> GAMGMNGIDDLLNINDRIKQVQNERNELASKLQNLKQSLASNDTGGGSGGGSDSSDLLQREAILANELNILDNLKTFLNLIKEVKTNLNILELENCYYSLQSLRKKMRNNAAYLKQSFNFQQSISTYVDTLHLELVSTLYKILTNGFWKITENSIQFTPTVEWGKDKVHIEYDTFMDFVAQQYFPKGSLDNQAWFILDMTSADSQEQVRAKLNTIMKEYMNLSRIVSMIKNSIFISGKEISYENEKNILVFSKSSSHGQHCVSTVLTSFEAVCDFMLDGLAFRDRKTLSYELGPLFNTEFTKFVKNNASIILE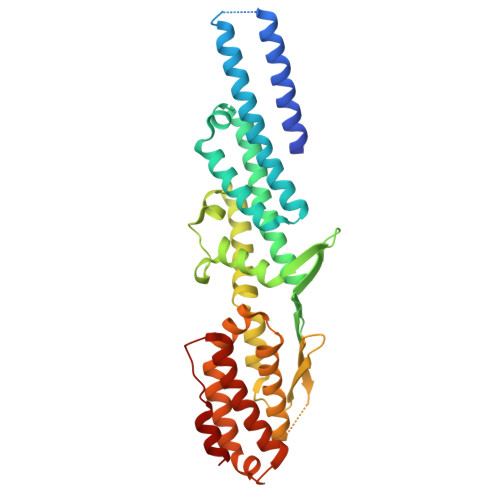SLDSPLKNLVSVINNKLTRLVAKSEVTNWTHSGKEIQDLLMN> MSLASLPISNFFTFNHQSTLFTKVKNFMGVKHIGDCMKALINGTIYTSFSPVKKVSGLVISNERVLYAGDSSTALRIAELAGGEIIDLKGKFVMPAFFDSHLHLDELGMSLEMVDLRGVKSMEELVERVKKGRGRIIFGFGWDQDELGRWPTREDLDVIDRPVFLYRRCFHVAVMNSKMIDLLNLKPSKDFDESTGIVRERALEESRKIINEKILTVKDYKHYIESAQEHLLSLGVHSVGFMSVGEKALKALFELEREGRLKMNVFAYLSPELLDKLEELNLGKFEGRRLRIWGVKLFVDGSLGARTALLSEPYTDNPTTSGELVMNKDEIVEVIERAKPLGLDVAVHAIGDKAVDVALDAFEEAEFSGRIEHASLVRD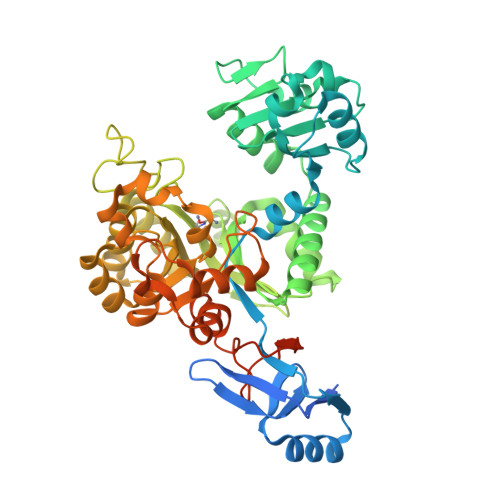DQLERIKELKVRISAQPHFIVSDWWIVNRVGEERAKWAYRLKTLSSITKLGFSTDSPIEPADPWVSIDAAVNRYVVDPGERVSREEALHLYTHGSAQVTLAEDLGKLERGFRAEYIILDRDPLKEMKGIITITTDPNSSSVDKLAAALEHHHHHH> GPLGSPEFDNNIENIGDGAEVVKRTEDTSSDKWGVTQNIQFDFVKDKKYNKDALILKMQGFINSKTTYYNYKNTDHIKAMRWPFQYNIGLKTNDPNVDLINYLPKNKIDSVNVSQTLGYNIGGNFNSGPSTGGNGSFNYSKTISYNQQNYISEVEHQNSKSVQWGIKANSFITSLGKMSGHDPNLFVGYKPYSQNPRDYFVPDNELPPLVHSGFNPSFIATVSHEKGSGDTSEFEITYGRNMDVTHATRRTTHYGNSALEGSRIHNAFVNRNYTVKYEVNWKTHEIKVKGHN

With the exception of α-hemolysin, which is homo-heptameric, leukotoxins are bipartite toxins, formed by the non-covalent association of two distinct proteins, a class S and a class F component of approximately 31 and 34 kDa, respectively, into a likely octameric species. Panton-Valentine leukocidin (PVL) is associated with necrotizing skin infections, such as boils, and plays an important role in the poor prognosis of necrotizing pneumonia. Two additional structural domains are also found: the rim domain anchors the protein to the membrane surface, while the stem domain, closely apposed to the core β-sandwich in the soluble form, contributes two β-strands to the pore β-barrel. Since the binding of LukS-PV to the membrane is a saturable process, the necessary presence of a LukS-PV receptor on the cell surface was thus proposed. This was recently confirmed by Spaan et al. who showed that the C5a receptor is required for the binding of LukS-PV to human neutrophils.

The mutants exhibiting significantly decreased binding abilities with respect to wild-type LukS-PV were: R73A, Y184A, T244A, H245A, and Y250A, with Ki values ranging from 1.8 to 6.2 nM, i.e. a 69- to 238-fold increase compared to the Ki value of wild-type LukS-PV. Four LukS-PV mutants (R73A, Y184A, T244A, and Y250) displayed significant alterations for all measured parameters, i.e. at least 50-fold decrease in affinity for hPMN membranes, 2-fold decrease in the slope of Ca2+ influx and 2- to 10-fold reduction in pore-forming capacity. The Y250A mutant crystallized in 5% PEG 6000, 0.1 M sodium citrate, pH 4.0. Crystals were orthorhombic, space group P21212, with cell parameters a = 85.30 Å, b = 84.29 Å and c = 38.09 Å and 1 molecule per asymmetric unit. Crystals diffracted up to 1.55 Å. In the case of the rim domain, wild-type LukS-PV and mutants T244A, Y246A and N248A displayed only small differences, with r.m.s. deviations comprised between 0.20 Å and 0.30 Å, whereas the structure of the rim domain of the Y184A and Y250A mutants were markedly different, with r.m.s. deviations of 1.10 Å and 1.28 Å, respectively, when compared to the wild-type LukS-PV structure. Of particular note, the rim region was generally associated with weak electron density, and could not be completely built in most structures, except in the case of the Y250A mutant. In the Y250A mutant structure, the removal of the tyrosine side chain allowed the displacement of the N248 side chain, which in turn drove the reorganization of residues R241–Y250. Space was therefore provided for the displacement of the V179–Q186 loop, which adopted a conformation close to that observed in the case of the Y184A mutant. For both Y184A and Y250A mutants, crystallization was achieved in different conditions than those for wild-type LukS-PV and the other mutants, resulting in a different crystal packing.L-2-AMINO-6-METHYLENE-PIMELIC 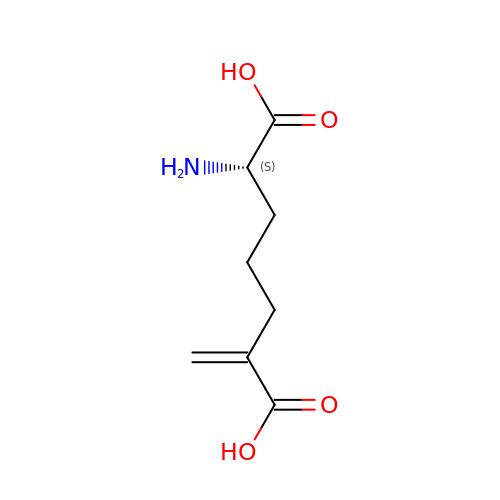ACID | C8 H13 N O4 | SGAIRWMSXVAPOO-LURJTMIESA-N5-azanyl-3-[1-[[(3~{R})-1-(phenylmethyl)piperidin-3-yl]methyl]indol-6-yl]-1~{H}-pyrazole-4-carbonitrile | C25 H26 N6 | 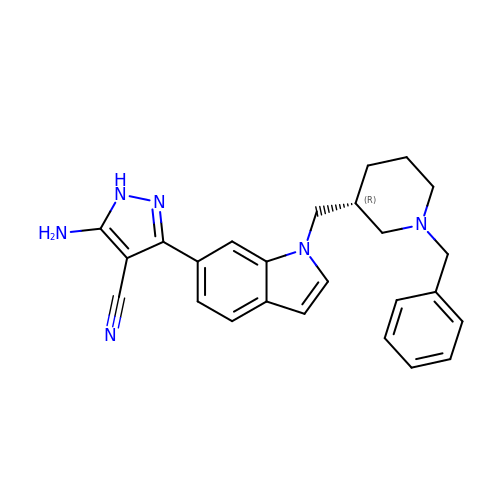RLAAKYCZJLWQDL-LJQANCHMSA-N> MADYQGKNVVIIGLGLTGLSCVDFFLARGVTPRVMDTRMTPPGLDKLPEAVERHTGSLNDEWLMAADLIVASPGIALAHPSLSAAADAGIEIVGDIELFCREAQAPIVAITGSNGKSTVTTLVGEMAKAAGVNVGVGGNIGLPALMLLDDECELYVLELSSFQLETTSSLQAVAATILNVTEDHMDRYPFGLQQYRAAKLRIYENAKVCVVNADDALTMPIRGADERCVSFGVNMGDYHLNHQQGETWLRVKGEKVLNVKEMKLSGQHNYTNALAALAL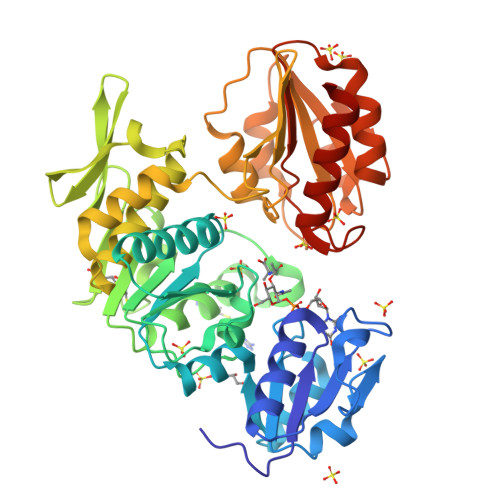ADAAGLPRASSLKALTTFTGLPHRFEVVLEHNGVRWINDSKATNVGSTEAALNGLHVDGTLHLLLGGDGKSADFSPLARYLNGDNVRLYCFGRDGAQLAALRPEVAEQTETMEQAMRLLAPRVQPGDMVLLSPACASLDQFKNFEQRGNEFARLAKELGGHHHHHH>[2x]SEEITDGVNNMNLATDSQKKNRIQVSNTKKPLFFYVNLAKRYMQQYNDVELSALGMAIATVVTVTEILKNNGFAVEKKIMTSIVDIKDDARGRPVQKAKI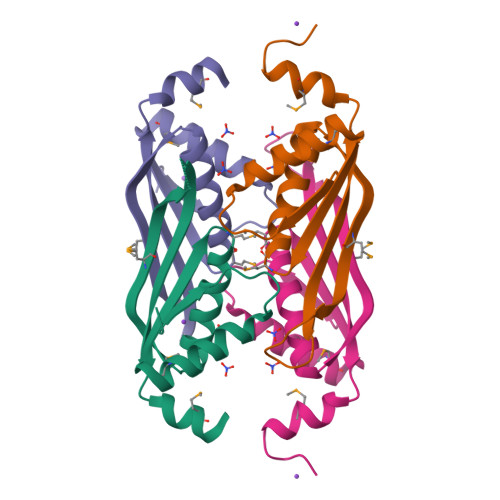EITLVKSEKFDELMAAANEEKEDAETQVQN>[4x]MTENIHKHRILILDFGSQYTQLVARRVRELGVYCELWAWDVTEAQIRDFNPSGIILSGGPESTTEENSPRAPQYVFEAGVPVFGVCYGMQTMAMQLGGHVEASNEREFGYAQVEVVNDSALVRGIEDALTADGKPLLDVWMSHGDKVTAIPSDFITVASTESCPFAIMANEEKRFYGVQFHPEVTHTRQGMRML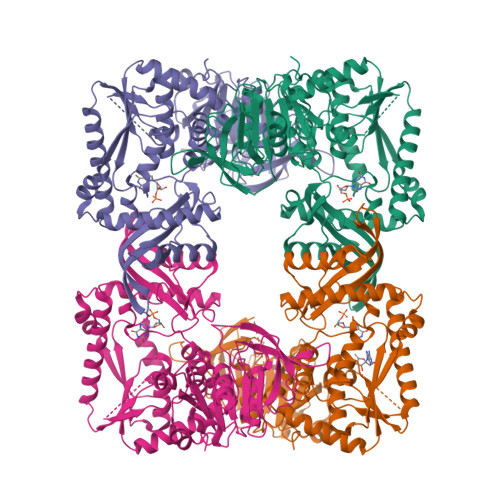ERFVRDICQCEALWTPAKIIDDAVARIREQVGDDKVILGLSGGVDSSVTAMLLHRAIGKNLTCVFVDNGLLRLNEAEQVLDMFGDHFGLNIVHVPAEDRFLSALAGENDPEAKRKIIGRVFVEVFDEEALKLEDVKWLAQGTIYPDVIESAASATGKAHVIKSHHNVGGLPKEMKMGLVEPLKELFKDEVRKIGLELGLPYDMLYRHPFPGPGLGVRVLGEVKKEYCDLLRRADAIFIEELRKADLYDKVSQAFTVFLPVRSVGVMGDGRKYDWVVSLRAVETIDFMTAHWAHLPYDFLGRVSNRIINEVNGISRVVYDISGKPPATIEWE> GGGDDN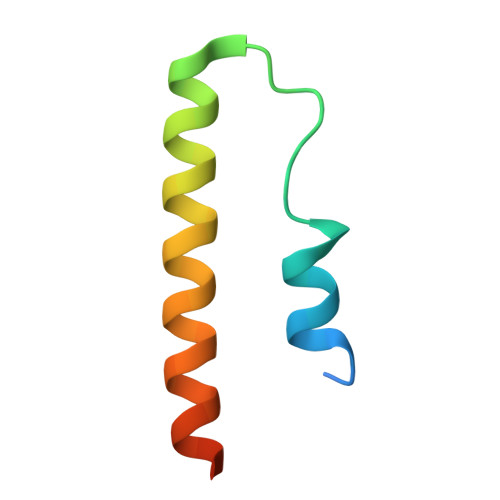TFNFSWKVFCSWDYLIGNPETADNKFNSITMNFKEAIIEERAAQVEENI Luffaculin 1 is a new type 1 ribosome-inactivating protein (RIP) isolated from the seeds of Luffa acutangula. The ribosome-inactivating proteins (RIPs) are RNA N-glycosidases that inactivate ribosome by cleaving a single N-C glycosidic bond between adenine and ribose at A4324 in the 28S eukaryotic mammalian rRNA or at A2660 in the 23S Escherichia coli rRNA. The removal of one adenine from rRNA by RIPs prevents the binding of elongation factor II (EF-2) to the 60S subunit, resulting in the termination of protein translation. Luffaculin 1 not only possesses rRNA N-glycosidase activity as expected, but also inhibits proliferation of tumor cells, induces apoptosis and differentiation on tumor cells.

Here, we report the high resolution (1.4 Å) crystal structure of luffaculin 1 and the protein sequence derived from this crystal structure. The crystals of luffaculin 1 belong to space group P1 and diffract to 1.4 Å resolution with synchrotron X-ray radiation. The crystals of luffaculin 1 contain two enzyme molecules (A and B) in the asymmetric unit. A comparison of molecules A and B shows that the overall structures of these two molecules are almost identical with rmsd of 0.181 Å for 221 Cα atoms. The structure of luffaculin 1 contains two domains: a large N-terminal domain composed of eight α-helices and eight β-strands, and a smaller C-terminal domain consisting of two α-helices (α9 and α10) and two β-strands (β9 and β10). The electron density of luffaculin 1 clearly indicated the existence of two well-defined N-acetylglucosamines (NAGs), each covalently linked to an Asn residue at positions 77 and 84, respectively. Although the sequence of luffaculin 1 is not yet known, the high resolution of electron density, combined with the known sequence of homolog luffin a, has allowed us to undertake an 'X-ray sequencing' method with a high degree of confidence. The existence of two independent luffaculin 1 molecules in the asymmetric unit allows the cross-validation of this X-ray sequence, further increasing the reliability of the sequence assignment. By using electron density and evaluation of chemical environment, 86% of residues were assigned with confidence.

>[2x]DVSFSLSGSSSTSYSKFIGALRKALPSNGTVYNITLLLSSASGASRYTLMKLSNYDGKAITVAIDVTNVYIMGYLVNSTSYFFNESDAKLASQYVFAGSTIVTLPYSGNYEKLQTAAGKIREKIPLGFPALDSAITTLFHYDSTAAAAAFLVIIQTTAESSRFKYIEGQIIMRISKNGVPSLATISLENEWSALSKQIQLAQTNNGTFKTPVVIMDAGGQRVEIGNVGSKVVTKNIQLLLN8,9-DIHYDRO-9-HYDROXY-AFLATOXIN B1 | C17 H14 O7 | 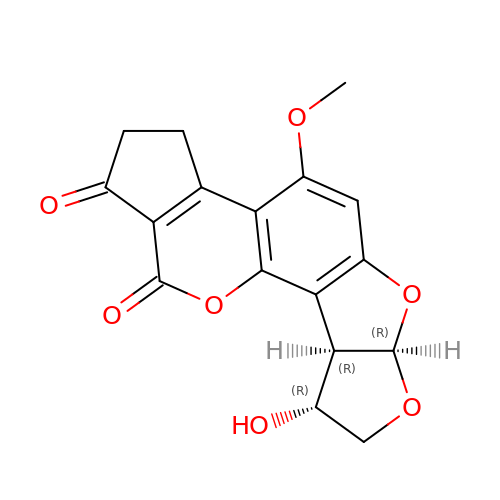GACWFTLPANAFAK-GVLSTKRJSA-N>MGMKTYDLIVIGFGKAGKTLAKYAASTGQHVAVIEQSPKMYGGTSINIGCIPSKTLVHDGLEGKSFEASYNRKNDVVNALNNKNYHLLADDNNIDVLDFKAQFKSNTEVNLLDQHDDIVDSITAPHIIINTGATSVIPNIKGLDQAKHVFDSTGLLNISYQPKHLVIVGGGYIALEFASMFANLGSKVTVLERGESFMPREDQDVVAYGITDLENKGIALHTNVETTELSSDNHHTTVHTNVDNFEADAVLLAIGRKPNTDLALENTDIELGDRGEIKVNAHLQTTVPHIYAAGDVKGGLQFTYISLDDYRIIKSALYGNQSRTTDNRGSVPYTVFIDPPLSRVGLTSKEAAAQHYDYTEHQLLVSAIPRHKINNDPRGLFKVVINNENNMILGATLYGKQSEELINIIK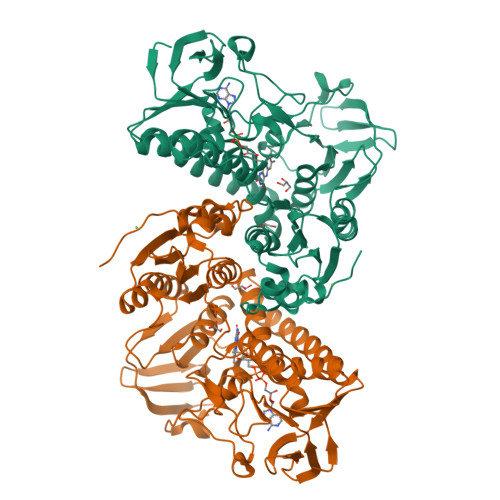LAIDQNIPYTVLRDNIYTHPTMAESFNDLFNFHHHHHH[2x]>[3x]MKMYDAYISYVNNENDRKFVNFILKPHLENKYSHKLLLNNTNILPGAEPS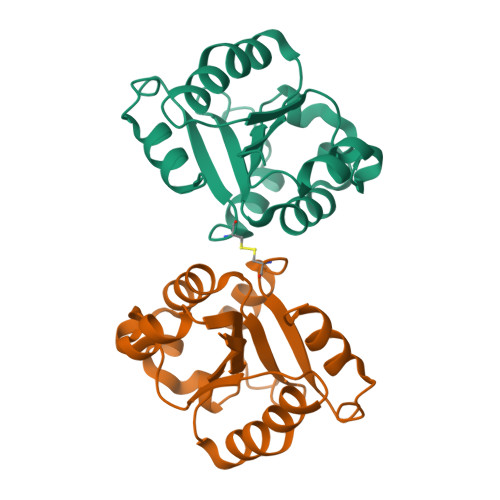AELLMNISRCQRLIVVLSQSYLEQEWCTTNFRQGLWHLIELSRKPIFIIFQSQQKQISQDISQQLRQHQPCITMITWGAHSMTPSSGFWKELALVMPRKHHHHHH> SGVDDDMACHKIPVEADFLYAYSTAPGYYSWRNSKDGSWFIQSLCAMLKQYA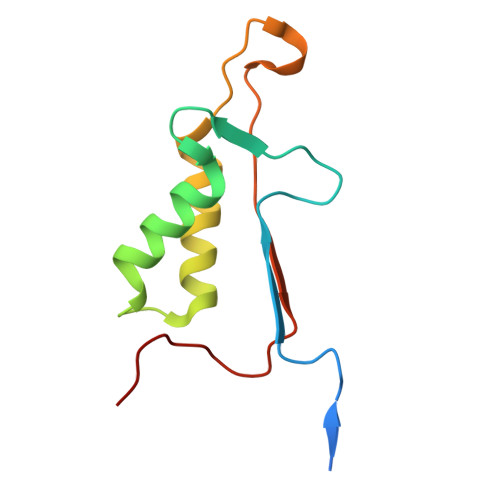DKLEFMHILTRVNRKVATEFESFSFDATFHAKKQIPCIVSMLTKELYFYHH> TLTEDLDAPQDTGNIENGAADNSPQPRTTFDYTGNPLPPDTKLENFFSFYRLL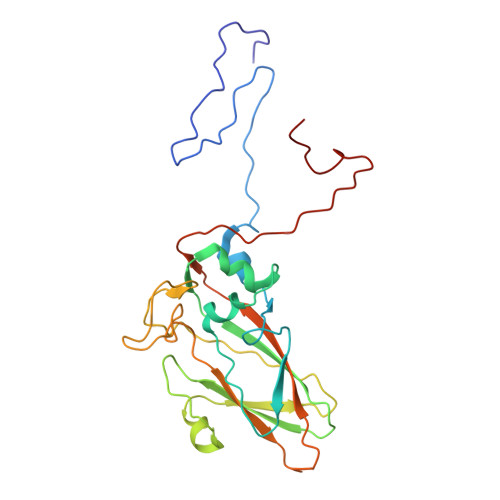PMGGSGAPSLSFPADEGTIIPLDPINWLKGADVSGIAAMLSCFTYIAADLRITLRFSNPNDNPATMLVAFAPPGATIPLKPTRQMLSNFYMAEVPVSAATSTMVSFSIPYTSPLSAIPTSYFGWEDWSGTNFGQLSSGSWGNLMLIPSLSVDSAIPFDFQLSCWVAFGNFKAWVPRPPPPLPPLPTPAANAERTVAVIKQ> GMVPISPIETVPVKLKPGMDGPKVKQWPLTEEKIKALVEICTEMEKEGKISKIGPENPYNTPVFAIKKKDSTKWRKLVDFRELNKRTQDFWEVQLGIPHPAGLKKKKSVTVLDVGDAYFSVPLDEDFRKYTAFTIPSINNETPGIRYQYNVLPQGWKGSPAIFQSSMTKILEPFAAQNPDIVIYQYMDDLYVGSDLEIGQ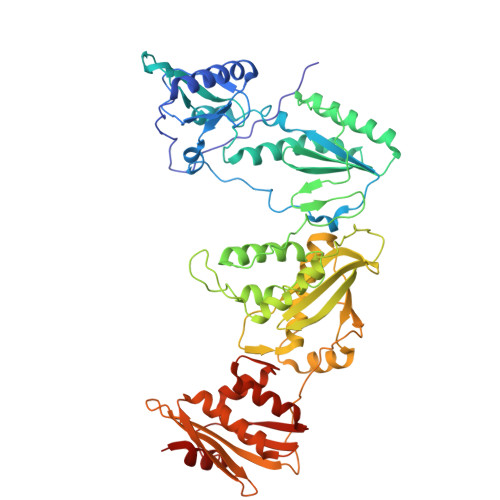HRTKIEELRQHLLRWGLTTPDKKHQKEPPFLWMGYELHPDKWTVQPIVLPEKDSWTVNDIQKLVGKLNWASQIYPGIKVRQLSKLLRGTKALTEVIPLTEEAELELAENREILKEPVHGVYYDPSKDLIAEIQKQGQGQWTYQIYQEPFKNLKTGKYARMRGAHTNDVKQLTEAVQKITTESIVIWGKTPKFKLPIQKETWETWWTEYWQATWIPEWEFVNTPPLVKLWYQLEKEPIVGAETFYVDGAANRETKLGKAGYVTNKGRQKVVPLTNTTNQKTELQAIYLALQDSGLEVNIVTDSQYALGIIQAQPDKSESELVNQIIEQLIKKEKVYLAWVPAHKGIGGNEQVDKLVSAG>NFEEPADAIEYRQAAFGLIAYNFGDMGAMLKGKKPFDAAVFSTRADNVAALSKIPHEGFIAGSDKGDTEALAKIWQ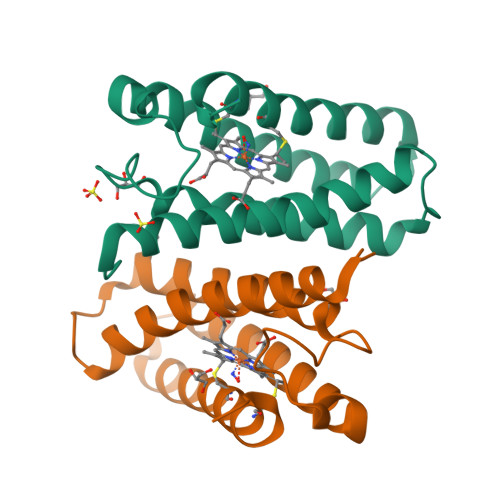DKADFDSKMTAFQDNAAALAVAAKSSDQNNIKQAFANTGKSCKGCHDVYKKD[2x]>[2x]MAGQLLFANFNQDNTSLAVGSKSGYKFFSLSSVDKLEQIYECTDTEDVCIVERLFSSSLVAIVSLKAPRKLKVCHFKKGTEI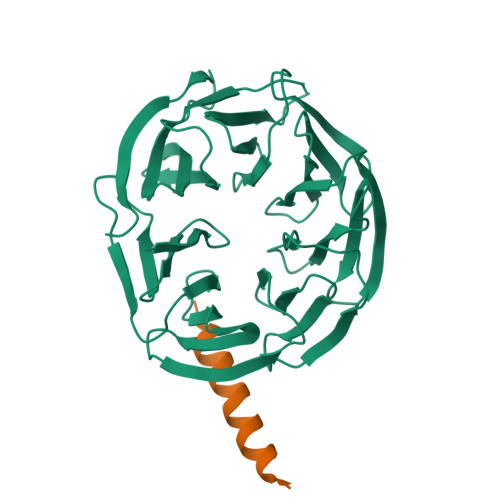CNYSYSNTILAVKLNRQRLIVCLEESLYIHNIRDMKVLHTIRETPPNPAGLCALSINNDNCYLAYPGSATIGEVQVFDTINLRAANMIPAHDSPLAALAFDASGTKLATASEKGTVIRVFSIPEGQKLFEFRRGVKRCVSICSLAFSMDGMFLSASSNTETVHIFKLETVGSGSFNQGRAFATVRLPFCGHKNICSLATIQKIPRLLVGAADGYLYMYNLDPQEGGECALMKQHRLDGSLET;>[2x]YAENEKDSRRRQARLQKELAEAAKE> MSTHRPFQLTHGSIEHTLLVPNDLFFNYSQLKDEFIKTLPEPTEGFAGDDEPSSPAELYGKFIGFISNAQFPQIVELSLKDFESRFLDNNNDNIHSFAVKLLDDETYPTTIAKVKENIVKNYYKAVKSINKVESNLLYHCKHDAKLVAIFGGQGNTDDYFEELRELYTLYQGLIEDLLVSIAEKLNQLHPSFDKIYTQGLNILSWLKHPETTPDQDYLLSVPVSCPVICVIQLCHYTITCKVLGLTPGEFRNSLKWSTGHSQGLVTAVTIAASDSWDSFLKNSLTAVSLLLFIGSRCLSTYPRTSLPPTMLQDSLDNGEGRPSPMLSVRDLSIKQVEKFIEQTNSHLPREKHIAISLINGARNLVLSGPPESLYGFNLNLRNQKAPMGLDQSRVPFSERKLKCSNRFLPIFAPFHSHLLADATELILDDVKEHGLSFEGLKIPVYDTFDGSDFQALKEPIIDRVVKLITELPVHWEEATNHKATHILDFGPGGVSGLGVLTHRNKEGTGARIILAGTLDSNPIDDEYGFKHEIFQTSADKAIKWAPDWLKELRPTLVKNSEGKIYVKTKFSQLLGRAPLMVAGMTPTTVNTDIVSASLNAGYHIELAGGGYFSPVMMTRAIDDIVSRIKPGYGLGINLIYVNPFMLQWGIPLIKDLREKGYPIQSLTIGAGVPSIEVATEYIEDLGLTHLGLKPGSVDAISQVIAIAKAHPTFPIVLQWTGGRGGGHHSFEDFHQPIIQMYSKIRRCSNIVLVAGSGFGSDEDTYPYLSGYWSEKFNYPPMPFDGVLFGSRVMTSKESHTSLAAKKLIVECKGVPDQQWEQTYKKPTGGIITVRSEMGEPIHKIATRGVMFWKELDDTIFNLPKNKLLDALNKKRDHIIKKLNNDFQKPWFGKNANGVCDLQEMTYKEVANRLVELMYVKKSHRWIDVSLRNMYGDFLRRVEERFTSSAGTVSLLQNFNQLNEPEQFTADFFEKFPQAGKQLISEEDCDYFLMLAARPGQKPVPFVPVLDERFEFFFKKDSLWQSEDLESVVDEDVQRTCILHGPVASQYTSKVDEPIGDILNSIHEGHIARLIKEEYAGDESKIPVVEYFGGKKPASVSATSVNIIDGNQVVYEIDSELPNKQEWLDLLAGTELNWLQAFISTDRIVQGSKHVSNPLHDILTPAKHSKVTIDKKTKKLTAFENIKGDLLPVVEIELVKPNTIQLSLIEHRTADTNPVALPFLYKYNPADGFAPILEIMEDRNERIKEFYWKLWFGSSVPYSNDINVEKAILGDEITISSQTISEFTHAIGNKCDA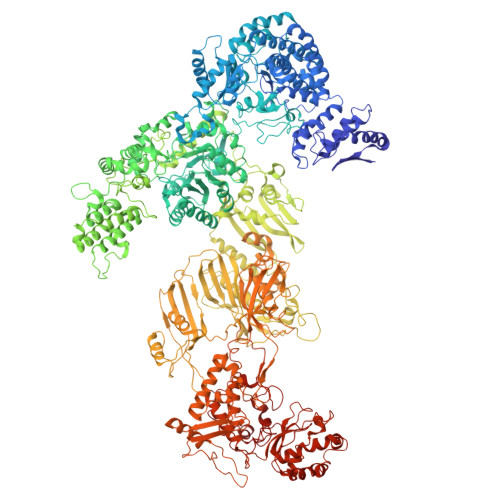FVDRPGKATLAPMDFAIVIGWKAIIKAIFPKSVDGDLLKLVHLSNGYKMITGAAPLKKGDVVSTKAEIKAVLNQPSGKLVEVVGTIYREGKPVMEVTSQFLYRGEYNDYCNTFQKVTETPVQVAFKSAKDLAVLRSKEWFHLEKDVQFDVLTFRCESTYKFKSANVYSSIKTTGQVLLELPTKEVIQVGSVDYEAGTSYGNPVTDYLSRNGKTIEESVIFENAIPLSSGEELTSKAPGTNEPYAIVSGDYNPIHVSRVFAAYAKLPGTITHGMYSSASIRALVEEWAANNVAARVRAFKCDFVGMVLPNDTLQTTMEHVGMINGRKIIKVETRNVETELPVLIGEAEIEQPTTTYVFTGQGSQEQGMGMELYNSSEVAREVWDKADRHFVNNYGFSILDIVQNNPNELTIHFGGAKGRAIRDNYIGMMFETIGEDGALKSEKIFKDIDETTTSYTFVSPTGLLSATQFTQPALTLMEKAAYEDIKSKGLIPSDIMFAGHSLGEYSALSSLANVMPIESLVDVVFYRGMTMQVAVPRDELGRSNYGMVAVNPSRVSATFDDSALRFVVDEVANKTKWLLEIVNYNVENQQYVAAGDLRALDTLTNVLNVLKINKIDIVKLQEQMSIEKVKEHLYEIVDEVAAKSLAKPQPIDLERGFAVIPLKGISVPFHSSYLMSGVKPFQRFLCKKIPKSSVKPQDLIGKYIPNLTAKPFELTKEYFQSVYDLTKSEKIKSILDNWEQYE> EAEAHHHHHHLANTSAHDFSYLKFVYNATDTSLEGSYDYIVIGGGTSGCPLAATLSEKYKVLLLERGTIATEYPNTLTADGFAYNLQQQDDGKTPVERFVSEDGIDNVRARILGGTTIINAGVYARANISFYSQTGIEWDLDLVNKTYEW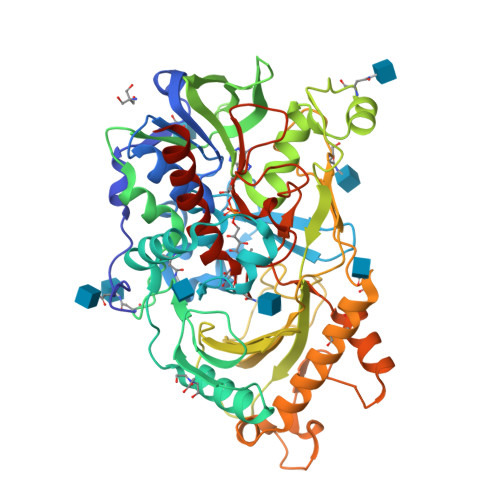VEDAIVVKPNNQSWQSVIGEGFLEAGILPDNGFSLDHEAGTRLTGSTFDNNGTRHAADELLNKGDPNNLLVAVQASVEKILFSSNTSNLSAIGVIYTDSDGNSHQAFVRGNGEVIVSAGTIGTPQLLLLSGVGPESYLSSLNITVVQPNPYVGQFVYDNPRNFINILPPNPIEASVVTVLGIRSDYYQVSLSSLPFSTPPFSFFPTTSYPLPNSTFAHIVSQVPGPLSHGSVTLNSSSDVRIAPNIKFNYYSNSTDLANCVSGMKKLGDLLRTKALEPYKARDVLGIDGFNYLGVPLPENQTDDASFETFCLDNVASYWHYHGGSLVGKVLDDSFRVMGIKALRVVDASTFPYEPNSHPQGFYLMLGRYVGLQILQERSIRLEAIHNIQESM> GSMNTIITHP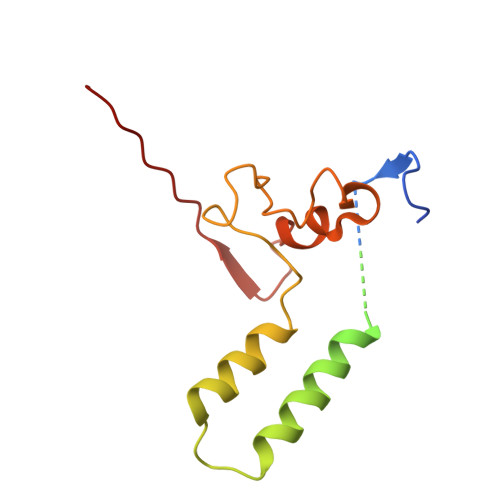GKMELVYVSDSDDSSSDNDSLTDLESLSSGESNEIKVTNDLDTSAEKDQIQAGKWFDPVLDWRKSDRELTKNILWRIADKTTYDKETITDLIEQGIPKHSYLSGNPLTSVTNDICSVENYETSSAFFYQQVHKKDRLQYLPLYAVSTFE> APPKTTVRWCTISSAEEKKCNSLKDHMQQERVTLSCVQKATYLDCIKAISNNEADAISLDGGQVFEAGLAPYKLKPIAAEVYERSGGSTTSYYAVAVVKKGTDFMIKDLRGKTSCHTGLGRSAGWNIPIGTLIHREDIEWEGIESGISEQAVAKFFSASCVPGATIEQKLCRQCKGDAKTKCLRNGPYSGYSGAFQCLKDGKGDVAFVKHTTVQENAPEEKDEYELLCLDGSRQPVDSYKTCNWARVAAHAVVARDDSKIDDIWSFLGMQAYSLGVDTTSDFHLFGPPGKKDPVLKDLLFKDSAIMLKRVPELMDSQLYLGFEYYSAIQSLRKDQLTVGPRENKIQWCAVGKDEKSKCDRWSVVSNGEVECTILDDNKDCIVKITKGEADAISLDGGFVYTAGVCGLVPVVGESYEDETQCSKDEEQPAYYFAVAVVKKSSAITWNNLQGKKSC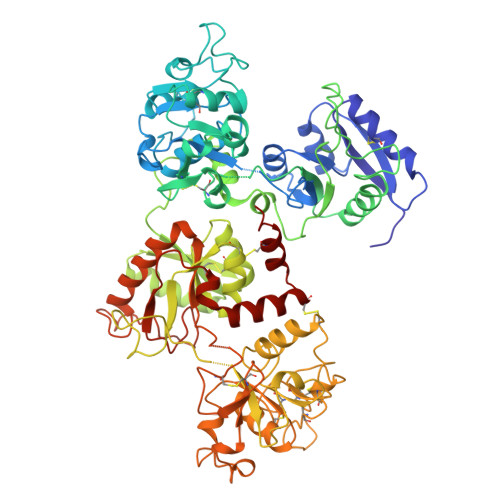HTAVGRTAGWNIPMGLIHNKTGSCDFDDYFSEGCAPGSPPNSRLCKLCQGSGENLLEKCVASSHEKYYGYTGALRCLVEQGDVAFIKHSTVGENVSGSNKDDWAKGLTRDDFELLCTNGKRAKTMDYKTCHLAKVPTHAVVARPEKANKIRELLEGQEKLFGLHGTEKERFMMFQSQTKDLLFKALTKCLVKLRQGITYKEFLGDEYYASVASLNTCNPSDLLQVCTFLEDK> DQNTEEMENLSDRVSQDTAGNTVTNTQSTVGRLVGYGTVHDGEHPASCADTASEKILAVERYYTFKVNDWTSTQKPFEYIRI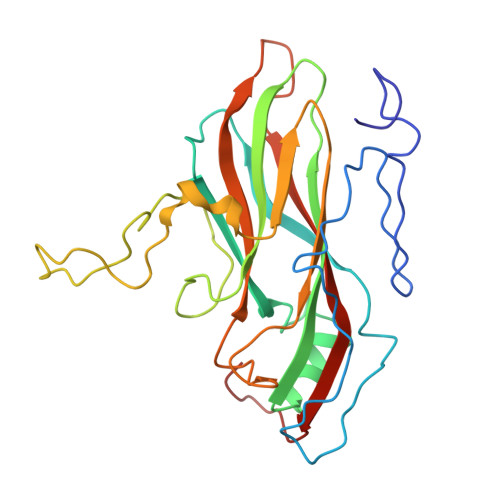PLPHVLSGEDGGVFGATLRRHYLVKTGWRVQVQCNASQFHAGSLLVFMAPEYPTLDVFAMDNRWSKDNLPNGTRTQTNRKGPFAMDHQNFWQWTLYPHQFLNLRTNTTVDLEVPYVNIAPTSSWTQHASWTLVIAVVAPLTYSTGASTSLDITASIQPVRPVFNGLRHEVLSRQ>GIGAVLKVLTTGLPALISWIKRKRQQ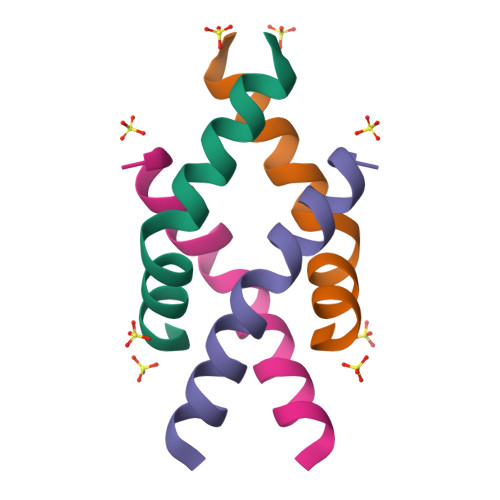X[4x]>NRPVFSQDVYRVRLPEDLPPGTTVLRLKAMDQDEGINAEFTYSFLGVANKAQFSLDPITGDIVTRQSLDFEEVEQYTIDVEAKDRGSLSSQCKVIIEVLDENDNRPEIIITSLSDQISEDSPSGTVVALFKVRDRDSGENAEVMCSLSGNNPFKIHSSSNNYYKLVTDSILDREQTPGYNVTITATDRGKPPLSSSTTITLNVADVNDNAPVFQQQAYLINVAENNQPGTSITQVKAWDPDVGSNGLVSYSIIASDLEPKALSSFVSVNQDSGVVYAQRAFDHEQ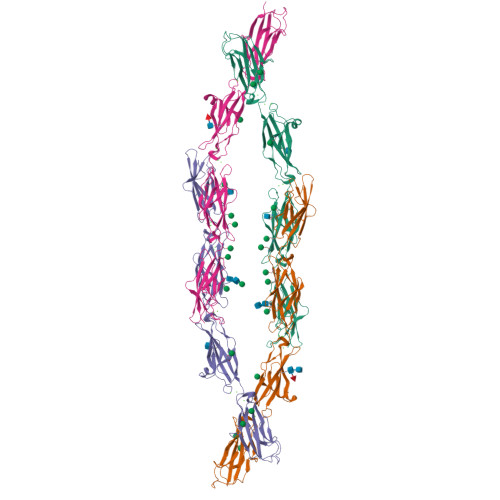IRSFQLTLQARDQGSPALSANVSMRVLVDDRNDNAPRVLYPTLEPDGSALFDMVPRAAEPGYLVTKVVAVDADSGHNAWLSYHVLQASDPGLFSLGLRTGEVRTARALSDKDAARQRLLVAVRDGGQPPLSATATLLLVFADSLQEHHHHHHHH[4x]>[2x]MTVPPTATHQPWPGVIAAYRDRLPVGDDWTPVTLLEGGTPLIAATNLSKQTGCTIHLKVEGLNPTGSFKDRGMTMAVTDALAHGQRAVLCASTGNTSASAAAYAARAGITCAVLIPQGKIAMGKLAQAVMHGAKIIQIDGNFDDCLELARK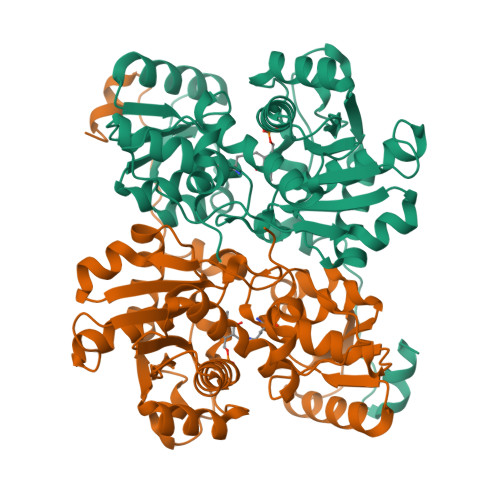MAADFPTISLVNSVNPVRIEGQKTAAFEIVDVLGTAPDVHALPVGNAGNITAYWKGYTEYHQLGLIDKLPRMLGTQAAGAAPLVLGEPVSHPETIATAIRIGSPASWTSAVEAQQQSKGRFLAASDEEILAAYHLVARVEGVFVEPASAASIAGLLKAIDDGWVARGSTVVCTVTGNGLKDPDTALKDMPSVSPVPVDPVAVVEKLGLA> MAKEVVEVLVTGGRATAGPPLGPAIGPLGVNVMQVVKEINEKTKDYEGM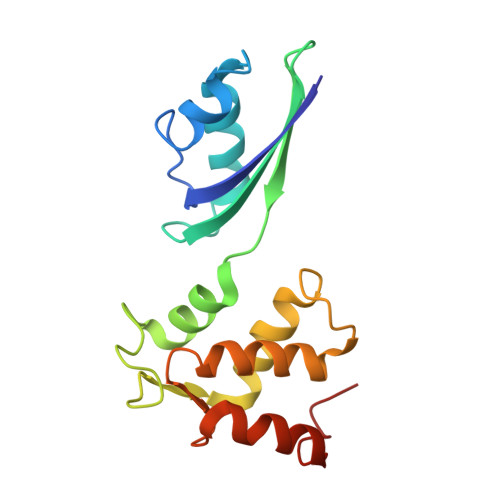QVPVKVIVDTETRKFEIEVGIPPTTALIKKELGIETAAHEPRHEVVGNLTLEQVIKIAKMKKDAMLSYTLKNAVKEVLGTCGSMGVTVEGKDPKEVQKEIDAGVYDEYFKEE> SNAMKKTLILGATPETNRYAY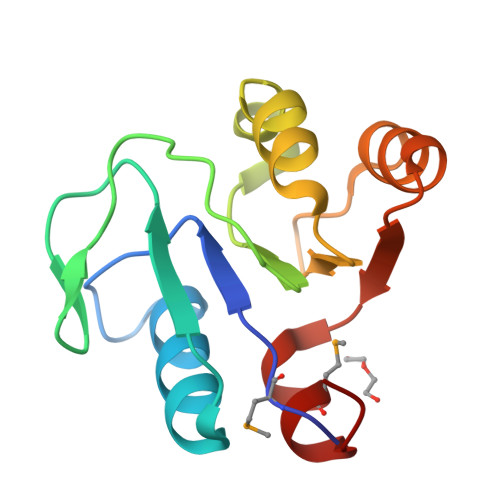LAAERLKSHGHEFIPVGRKKGEVLGKTIINERPVIEGVDTVTLYINPQNQLSEYNYILSLKPKRVIFNPGTENEELEEILSENGIEPVIGCTLVMLSAGTF>GSHMHTLYAPGGYDIMGYLIQIMNRPNPQVELGPVDTSCALVLCDLKQKDTPIVYASEAFLYMTGYSNAEVLGRNCRFLQSPDGMVKPKSTRKYVDSNTINTMRKAIDRNAEVQVEVVNFKKNGQRFVNFLTMI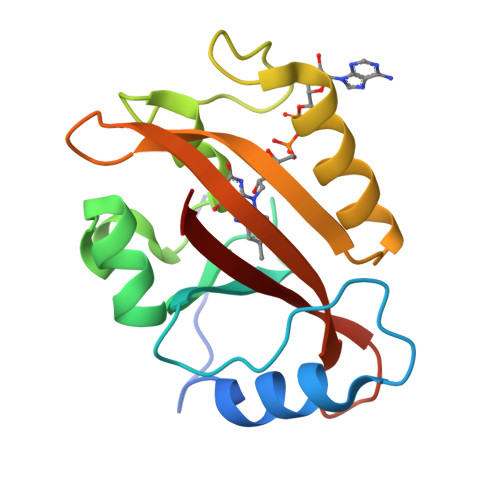PVRDETGEYRYSMGFQCETE[2x]> MESAGPGTGPQPPRTSGDFTPDTGVIAEMTGRPMRFDSDRYRPTDTYAEVACDKVCRAYEGLGADGGDRESLLAFLRDLTDPWGELPVGTPPEDACWVSIDGMPLETSVAWAGRKAGVRLSLESPRGPAKRRMEDGMALTRRLAGRPGVSVDPCLRVEDLFTDDDPQGYFTIAHAVAWTPGGHPRYKIFLNPAVRGREQAAARTEEAMIRLGLEQPWRALTEHLGGAYGPEHEPAALAMDLVPGDDFRVQVYLAHSGVSAEAIDAKSAVAADHVPGSFARALRGINGADDTPEWKRKPPVTAFSFGPGRAVPGATLYVPMIPVHGSDAAARDRVAAFLRSEGMDAVGYEAVLDAISDRSLPESHTQNFISYRGGDSPRFSVYLAPGVYREALEHHHHHH

Heterologous expression in Streptomyces lividans TK21 and an in vivo analysis revealed that TleC catalyses the ‘reverse' prenylation of the cyclic dipeptide (−)-indolactam V (1) at the C-7 position of the indole ring with geranyl pyrophosphate (GPP) (C10) to produce lyngbyatoxin A (2), with the C19R configuration, as in the case of LtxC15. MpnD also catalyses the ‘reverse' prenylation of 1 at the C-7 position, with DMAPP (C5) to yield pendolmycin (3). The overall structures of TleC and MpnD adopt the ABBA-fold, which consists of ten antiparallel β-strands assembled into a circular β-barrel, surrounded by a ring of solvent-exposed α-helices, as observed in the structures of indole PTs and aromatic PTs222324252627. In contrast to typical indole PTs that exhibit broad substrate specificities towards the prenyl acceptors but with strict specificities towards the prenyl donors, it is remarkable that the indolactam-specific TleC and MpnD exhibited unusually relaxed substrate specificities towards the prenyl donors and accepted different chain lengths (from C5 to C25) of prenyl pyrophosphate in vitro.

The gene cluster from S. blastmyceticus encodes an indolactam PT, TleC, which is a 42-kDa protein consisting of 391 amino acids that shares 40% and 38% identities with LtxC from the cyanobacterium Moorea producens and MpnD from the deep sea bacterium M. thermotolerans, respectively. S. blastmyceticus TleC and M. thermotolerans MpnD were heterologously expressed in Escherichia coli as His-tagged fusion proteins and purified to homogeneity by Ni-chelate affinity chromatography. TleC exhibited 23-fold higher kcat/KM value for the C10 prenylation activity over the C5 prenylation activity.> SKKILLTPRRRQRL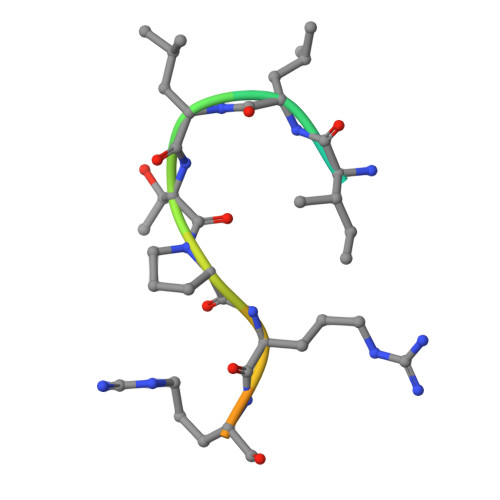S(2E)-2-{[(Z)-{3-hydroxy-2-methyl-5-[(phosphonooxy)methyl]pyridin-4(1H)-ylidene}methyl]imino}-3-phenylpropanoic 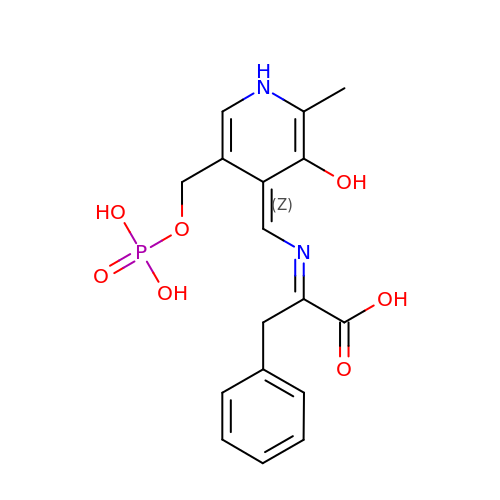acid | C17 H19 N2 O7 P | JRKRKLQVIAQBNI-NQHSUEJOSA-N6-[[(1~{R})-1-(4-chlorophenyl)-7-fluoranyl-1-[[1-(hydroxymethyl)cyclopropyl]methoxy]-3-oxidanylidene-5-(2-oxidanylpropan-2-yl)isoindol-2-yl]methyl]pyridine-3-carbonitrile | C29 H27 Cl F N3 O4 | 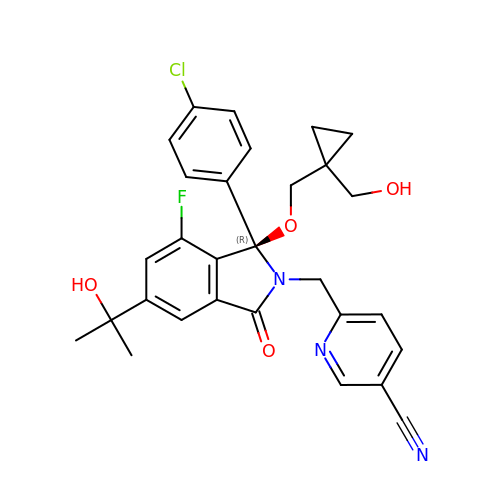GDVBWGYVVZIZIR-GDLZYMKVSA-N>[2x]MTGPILSGLDPRFERTLYAHVGKEGSWTLDYYLRHGGYETAKRVLKEKTPDEVIEEVKRSGLRGRGGAGFPTGLKWSFMPKDDGKQHYLICNADESEPGSFKDRYILEDVPHLLIEGMILAGYAIRATVGYIYVRGEYRRAADRLEQAIKEARARGYLGKNLFGTDFSFDLHVHRGAGAYICGEETALMNSLEGLRANPRLKPPFPAQSGLWGKPTTINNVETLASVVPIMERGADWFAQMGTEQSKGMKLYQISGPVKRPGVYELPMGTTFRELIYEWAGGPLEPIQAIIPGGSSTPPLPFTEEVLDTPMSYEHLQAKGSMLGTGGVILIPERVSMVDAMWNLTRFYAHESCGKCTPCREGVAGFMVNLFAKIGTGQGEEKDVENLEALLPLIEGRSFCPLADAAVWPVKGSLRHFKDQYLALAREKRPVPRPSLWR;>[2x]MGFFDDKQDFLEETFAKYPPEGRRAAIMPLLRRVQQEEGWIRPERIEEIARLVGTTPTEVMGVASFYSYYQFVPTGKYHLQVCATLSCKLAGAEELWDYLTETLGIGPGEVTPDGLFSVQKVECLGSCHTAPVIQVNDEPYVECVTRARLEALLAGLRAGKRLEEIELPGKCGHHVHEVEV;>[2x]MVRVKVNDRIVEVPPGTSVMDAVFHAGYDVPLFCSEKHLSPIGACRMCLVRIGLPKKGPDGKPLLNEKGEPEIQWQPKLAASCVTAVADGMVVDTLSDVVREAQAGMVEFTLLNHPLDCPTCDKGGACELQDRTVEYGLYEKYYQKGPLELPVYTRFEFTRRHVDKHHPLSPFVILDRERCIHCKRCVRYFEEVPGDEVLDFIERGVHTFIGTMDFGLPSGFSGNITDICPVGALLDLTARFRARNWEMEETPTTCALCPVGCGITADTRSGELLRIRAREVPEVNEIWICDAGRFGHEWADQNRLKTPLVRKEGRLVEATWEEAFLALKEGLKEARGEEVGLYLAHDATLEEGLLASELAKALKTPHLDFQGRTAAPASLFPPASLEDLLQADFALVLGDPTEEAPILHLRLSEFVRDLKPPHRYNHGTPFADLQIKERMPRRTDKMALFAPYRAPLMKWAAIHEVHRPGEEREILLALLGDKEGSEMVAKAKEAWEKAKNPVLILGAGVLQDTVAAERARLLAERKGAKVLAMTPAANARGLEAMGVLPGAKGASWDEPGALYAYYGFVPPEEALKGKRFVVMHLSHLHPLAERYAHVVLPAPTFYEKRGHLVNLEGRVLPLSPAPIENGEAEGALQVLALLAEALGVRPPFRLHLEAQKALKARKVPEAMGRLSFRLKELRPKERKGAFYLRPTMWKAHQAVGKAQEAARAELWAHPETARAEALPEGAQVAVETPFGRVEARVVHREDVPKGHLYLSALGPAAGLRVEGRVLVPAGGEA;>[2x]MREEFLEEIPLDAPPEEAKELRTEVMTLNVGPQHPSTHGVLRLMVTLSGEEVLEVVPHIGYLHTGFEKTMEHRTYLQNITYTPRMDYLHSFAHDLAYALAVEKLLGAVVPPRAETIRVILNELSRLASHLVFLGTGLLDLGALTPFFYAFRERETILDLFEWVTGQRFHHNYIRIGGVKEDLPEEFVPELKKLLEVLPHRIDEYEALFAESPIFYERARGVGVIPPEVAIDLGLTGGSLRASGVNYDVRKAYPYSGYETYTFDVPLGERGDVFDRMLVRIREMRESVKIIKQALERLEPGPVRDPNPQITPPPRHLLETSMEAVIYHFKHYTEGFHPPKGEVYVPTESARGELGYYIVSDGGSMPYRVKVRAPSFVNLQSLPYACKGEQVPDMVAIIASLDPVMGDVDR;>MRLERVLEEARAKGYPIEDNGLGNLWVVLPRERFKEEMAHYKAMGFNFLADIVGLDYLTYPDPRPERFAVVYELVSLPGWKDGDGSRFFVRVYVPEEDPRLPTVTDLWGSANFLEREVYDLFGIVFEGHPDLRKILTPEDLEGHPLRKDYPLGETPTLFREGRYIIPAEFRAALTGKDPGLTFYKGGSRKGYRSLWADLKKAREVKG[2x];>MALKDLFERDVQELEREGILFTTLEKLVAWGRSNSLWPATFGLACCAIEMMASTDARNDLARFGSEVFRASPRQADVMIVAGRLSKKMAPVMRRVWEQMPDPKWVISMGACASSGGMFNNYAIVQNVDSVVPVDVYVPGCPPRPEALIYAVMQLQKKVRGQAYNERGERLPPVAAWKRTRG[2x];>[2x]MSASSERELYEAWVELLSWMREYAQAKGVRFEKEADFPDFIYRMERPYDLPTTIMTASLSDGLGEPFLLADVSPRHAKLKRIGLRLPRAHIHLHAHYEPGKGLVTGKIPLTKERFFALADRAREALAFA;>MTLKALAQSLGITLKYLFSKPVTVPYPDAPVALKPRFHGRHVLTRHPNGLEKCIGCSLCAAACPAYAIYVEPAENDPENPVSAGERYAKVYEINMLRCIFCGLCEEACPTGAIVLGYDFEMADYEYSDLVYGKEDMLVDVVGTKPQRREAKRTGKPVKVGYVVPYVRPELEGFKAPTEGGKR[2x];>[2x]MAPIQEYVGTLIYVGVALFIGVAALLVGALLGPKKPGRAKLMPYESGNDPAGEVKRFPVHFYVVAMLFILFDVEVAFLWPYAVSAGGLGLYGFLGVLAFTLLLFVGFLYEWWKGVMRWH;>[2x]MTWSYPVDPYWMVALKALLVVVGLLTAFAFMTLIERRLLARFQVRMGPNRVGPFGLLQPLADAIKSIFKEDIVVAQADRFLFVLAPLISVVFALLAFGLIPFGPPGSFFGYQPWVINLDLGILYLFAVSELAVYGIFLSGWASGSKYSLLGSLRSSASLISYELGLGLALLAPVLLVGSLNLNDIVNWQKEHGWLFLYAFPAFLVYLIASMAEAARTPFDLPEAEQELVGGYHTEYSSIKWALFQMAEYIHFITASALIPTLFLGGWTMPVLEVPYLWMFLKIAFFLFFFIWIRATWFRLRYDQLLRFGWGFLFPLALLWFLVTALVVALDLPRTYLLYLSALSFLVLLGAVLYTPKPARKGGGA;>[2x]MSLLEGLALFLLLLSGVLVVTLRNAIHAALALILNFLVLAGVYVALDARFLGFIQVIVYAGAIVVLFLFVIMLLFAAQGEIGFDPLVRSRPLAALLALGVAGILAAGLWGLDLAFTQDLKGGLPQALGPLLYGDWLFVLLAVGFLLMAATVVAVALVEPGKASRAKEAEKREEVAR;>[2x]MSYLLTSALLFALGVYGVLTRRTAILVFLSIELMLNAANLSLVGFARAYGLDGQVAALMVIAVAAAEVAVGLGLIVAIFRHRESTAVDDLSELRG;>[2x]MALLGTILLPLLGFALLGLFGKRMREPLPGVLASGLVLASFLLGAGLLLSGGARFQAEWLPGIPFSLLLDNLSGFMLLIVTGVGFLIHVYAIGYMGGDPGYSRFFAYFNLFIAMMLTLVLADSYPVMFIGWEGVGLASFLLIGFWYKNPQYADSARKAFIVNRIGDLGFMLGMAILWALYGTLSISELKEAMEGPLKNPDLLALAGLLLFLGAVGKSAQIPLMVWLPDAMAGPTPVSALIHAATMVTAGVYLIARSSFLYSVLPDVSYAIAVVGLLTAAYGALSAFGQTDIKKIVAYSTISQLGYMFLAAGVGAYWVALFHVFTHAFFKALLFLASGSVIHALGGEQDVRKMGGLWKHLPQTRWHALIGALALGGLPLLSGFWSKDAILAATLTYPFGGVGFYVGALLVAVLTAMYAMRWFVLVFLGEERGHHHPHEAPPVMLWPNHLLALGSVLAGYLALPHPLPNVLEPFLKPALAEVEAHHLSLGAEWGLIALSAAVALLGLWAGFVFFQRKVFPAWYLAFEAASREAFYVDRAYNALIVNPLKALAEALFYGDRGLLSGYFGLGGAARSLGQGLARLQTGYLRVYALLFVLGALLLLGVMRW;>[2x]MVVLAVLLPVVFGALLLLGLPRALGVLGAGLSFLLNLYLFLTHPGGVAHAFQAPLLPGAGVYWAFGLDGLSALFFLTIALTVFLGALVARVEGRFLGLALLMEGLLLGLFAARDLLVFYVFFEAALIPALLMLYLYGGEGRTRALYTFVLFTLVGSLPMLAAVLGARLLSGSPTFLLEDLLAHPLQEEAAFWVFLGFALAFAIKTPLFPLHAWLPPFHQENHPSGLADALGTLYKVGVFAFFRFAIPLAPEGFAQAQGLLLFLAALSALYGAWVAFAAKDFKTLLAYAGLSHMGVAALGVFSGTPEGAMGGLYLLAASGVYTGGLFLLAGRLYERTGTLEIGRYRGLAQSAPGLAALALILFLAMVGLPGLSGFPGEFLTLLGAYKASPWLAALAFLSVIASAAYALTAFQKTFWEEGGSGVKDLAGAEWGFALLSVLALLLMGVFPGYFARGLHPLAEAFAKLLGGGA;>MTLAILAVFSVALTLLGFVLPPQGVKRATLLGLALALASLLLTWGKPFAFGPYAVDGVSQVFTLLALLGALWTVGLVRSGRFEFYLLVLYAALGMHLLASTRHLLLMLVALEALSLPLYALATWRRGQGLEAALKYFLLGALAAAFFLYGAALFYGATGSLVLGAPGEGPLYALALGLLLVGLGFKAALAPFHFWTPDVYQGSPTPVVLFMATSVKAAAFAALLRVAAPPEALALLVALSVVVGNLAALAQKEAKRLLAYSSIAHAGYMALALYTGNAQALGFYLLTYVLATGLAFAVLSQISPDRVPLEALRGLYRKDPLLGLAFLVAMLSLLGLPPLAGFWGKYLAFAEAARAGAWGVLVLALVTSAVSAYYYLGLGLAVFARPEETPFRPGPPWARAAVVAAGVLLLALGLLPGLVLPALAAGG[2x];>[2x]MVRVGMRAAPRVSLEALKAALGGLKLSEAKVYLITDWQDKRDQARYALLLHTGKKDLLVPDAFGPAFPGGEEALSELVGLLLAQGARRFYEAVVSPGEMTALLDLPPEELLKRVMAIANPTDPGIYLKRAA

Complex I (NADH:ubiquinone (UQ) oxidoreductase) is the first and the largest enzyme of the respiratory chain, catalysing the transfer of two electrons from NADH to UQ, coupled to the translocation of four protons across the bacterial or inner mitochondrial membrane. In bacterial complex I the 14 “core” subunits, necessary and sufficient for complex I function, are shared equally between the peripheral and membrane arms, together forming an L-shaped molecule. All known co-factors of complex I reside in the PA: the primary electron acceptor flavin-mononucleotide (FMN) is connected by the redox chain of seven Fe–S clusters to the quinone-binding site (Q-site) at the interface with the membrane domain. In this work we address this question by building and analyzing atomic structures of nine different conformational states of complex I, which were obtained by X-ray crystallography and single-particle cryo-EM.

The FMN is coordinated by subunit Nqo1 at the deep end of a solvent-exposed cavity that contains also the NADH-binding site. The binding of NADH relies on stacking and polar interactions. The nicotinamide ring is located in the inner region of the pocket, establishing a stacking interaction with FMN flavin ring while polar contacts with charged residues K2021 (suffix indicates subunit) and E1851 stabilize the diphosphate moiety. The adenosine ring is stabilized by stacking interactions with F701 and F2051. Binding of NADH per se had no major effect on the structure of complex I, as the crystal structure of the CXINADH shows a very high level of structural similarity to the crystal structure of the native state, CXIINT. However, this is true only after relatively short incubation times with NADH of up to about 30 min. Since at least three NADH oxidation cycles are required to fully reduce the redox chain in complex I33 and the rate of NADH diffusion into crystals during soaking is limited (probably at least to the scale of minutes), it is possible that these structures represent a partially reduced complex, where NADH is bound, but FMN and some of the reducible clusters in the chain are still oxidized. Importantly most regions around the Q-site show marginal changes in the CXINADH structure, with the exception of the key H384 flipping after extended incubation with NADH. In contrast to our original expectations, NADH binding and subsequent reduction of the enzyme does not lead to large conformational changes apart from flipping of H384 upon extended soaking, which likely plays a role in regulating Q access into the deep end of the cavity.> MIKEMIEDFISKGGLI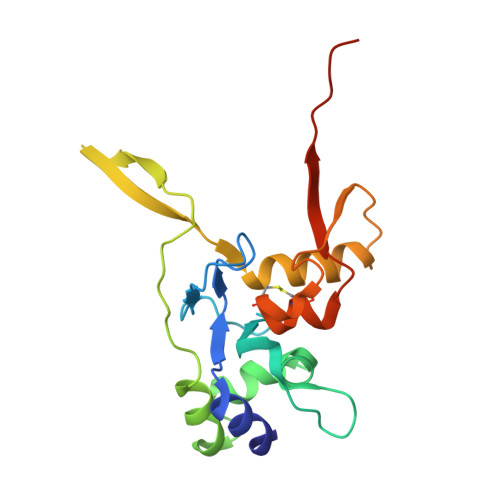FTHSGRYTNTNNSCFIFNKNDIGVDTKVDMYTPKSAGIKNEEGENLWQVLNKANMFYRIYSGELGEELQYLLKSCCTAKEDVTTLPQIYFKNGEGYDILVPIGNAHNLISGTEYLWEHKYYNTFTQKLGGSNPQNCTHACNKMRGGFKQFNCTPPQVEDNYNA> GPFTLDHAPRITLRMRSHR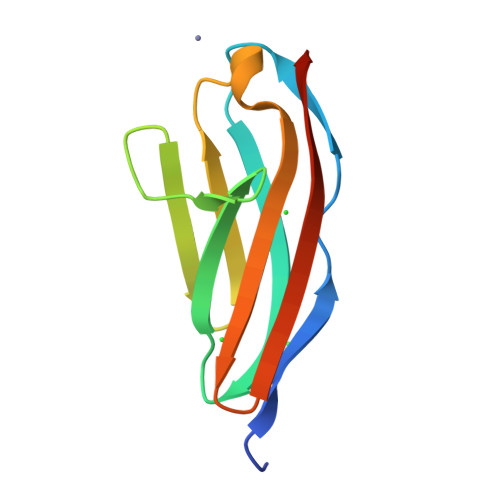VPCGQNTRFILNVQSKPTAEVKWYHNGVELQESSKIHYTNTSGVLTLEILDCHTDDSGTYRAVCTNYKGEASDYATLDVTGGDY>[2x]ISEFGSEPIDPSKLEFARALYDFVPENPEMEVALKKGDLMAILSKKDPLGRDS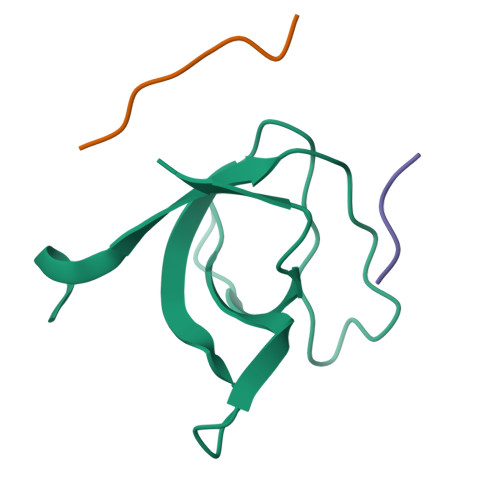DWWKVRTKNGNIGYIPYNYIEIIKRRK;>[3x]XEAMPPTLPHRDWKD>SYTLPSLPYAYDALEPHFDKQTMEIHHTKHHQTYVNNANAALESLPEFANLPVEELITKLDQLPADKKTVLRNNAGGHANHSLFWKGLKKGTTLQGDLKAAIERDFGSVDNFKAEFEKAAASRFGSGWAWLVLKGDKLAVVSTANQDSPLM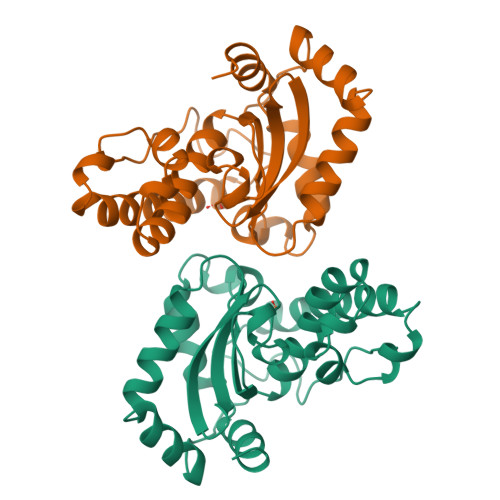GEAISGASGFPIMGLDVWEHAYYLKFQNRRPDYIKEFWNVVNWDEAAARFAAKK[2x]>[2x]NVHSNYTFIIAGGGISGLTLADRLTEDPRVTVLVIEAGPLDRGEDGILVPGAFSPWLYFWPGLVSTPQAGLNNRTVDVITAQVVGGGSTINAMVYLRGDKDDYDSWGALGNPGWSWNSMLPYFIKSETFTPPSPELAAAGNITWDGSIRGRSGPVNYSYPNYFFPGSENWWNAANEVGLPPVKDPMAGSKQGVFWIPSAIDARTMTRSHARRNHYDRVSSRPNYHILPSHLVSKILFRGKQAIGVSYIPTSGGNTTTNVYASKEITLAAGGLGTPKILQLSGIGPRKLLNELGIPVISDLPGVGQNLQDQPTLTIPYTFTNNVFPNTDSLTTNATYNAEQRALYDSSKQGAYTIVNSLSTNIGVMSLQRAAPKSYRQIIAAARARSASLSLPPGTDPAVIRGYQAQRNAILKQFENPNVGVGTVHWGTGSSALVYHLKPLSRGTVNIRSTNPLDAPEIDYRTGTDPIDAQVYTSLFRKNREIFNAPSMRVLGPSEAAPFGANLTTDEEIYAVMRELINPSNAHQCCTAAMMPKDMGGVVSSEQKVYGVQGLRVADISFWPFQLSGSPMATAYAGAERLADVIKKEHRLAGAPKSL

The FAD-dependent oxidoreductase from Chaetomium thermophilum (CtFDO) is a novel thermostable glycoprotein from the glucose–methanol–choline (GMC) oxidoreductase superfamily. However, CtFDO shows no activity toward the typical substrates of the family and high-throughput screening with around 1000 compounds did not yield any strongly reacting substrate. The structure of CtFDO reveals an unusually wide-open solvent-accessible active-site pocket with a unique His–Ser amino-acid pair putatively involved in enzyme catalysis. A series of six crystal structures of CtFDO complexes revealed five different subsites for the binding of aryl moieties inside the active-site pocket and conformational flexibility of the interacting amino acids when adapting to a particular ligand.

PESB interacts via a hydrogen bond with Asn562 and via WAS with flavin, His564 and Ser607 (‘in’ conformer). PESB is further stabilized by vdW interactions with FAD, Ala133, Val135, Leu399, His466, Leu474, Tyr476 and Asn562. The formic acid molecule makes the same interactions in S1 as in CtFDO:MAMB, and WAS (HOHA804 in chain A, HOHB817 in chain B) adopts an almost identical position as WAS in CtFDO:free (shifted by 0.2 and 0.5 Å for chains A and B, respectively). Subsite S2 of CtFDO was found to bind only aromatic moieties (the thiophene moiety of PESB). Different moieties of the bound compounds use the individual subsites differently. The CS, which is located in the narrow passage of the pocket, binds both aromatic (MAMB, the pyrrole of IPEA and the benzothiazoline of ABTS) and aliphatic (formic acid, PESB and IPEA) moieties. Ser607 in the ‘in’ conformation participates in binding the active-site water molecule (CtFDO:free and CtFDO:PESB), formic acid in the S1 subsite (CtFDO:MAMB, CtFDO:PESB and CtFDO:IPEA) and in the catalytic site (CtFDO:4NP).>[5x]MYSCRAVGVDA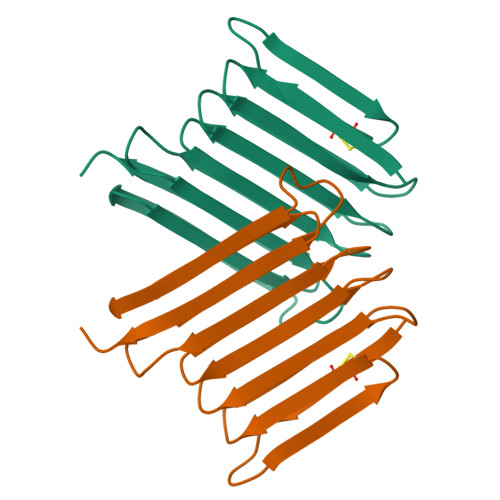STVTDVQGTCHAKATGPGAVASGTSVDGSTSTATATGSGATATSTSTGTGTATTTATSNAAATSNAIGQGTATSTATGTAAARAIGSSTTSASATEPTQTKTVSGPGAQTATAIAIDTATTTVTASLEHHHHHH> MGSSHHHHHHSSGLVPRGSHMQEQTAKEDVADSATSVGAIVSIEKAEKNFVITYASGKKAQISILNDHLFRYHLDPTGKFEEYPTPNDPKHVAKITAKTMADYGTQAFEQTNVTDSGNQFILENNGLKIIFEKESALMKVLDKKKNQVILEETAPLSFKNDKATQTLKQSSQENYFGGGTQNGRFTHKGTAIQIVNTNNWVDGGVASPNPFYWSTAGYGVVRNTWKPGNYDFGSHDPQTTTTTHEGTDFDAFYFFNDSSAGILKDYYELTGKPALMPEYGFYEAHLNAYNRDYWVKVAEGTAGAVKFEDGNFYKEYQPGDLGNLNGTLESLNGEKENYQFSARAVIDRYKKNDMPLGWFLPNDGYGAGYGQTDSLDGDVQNLKEFTDYAQANGVEVGLWTQSNLHPADPKNPKKGERDIAKEVSVAGVKALKTNVAWVGYGYSFGLNGVEDAANVFVKETDGAVRPM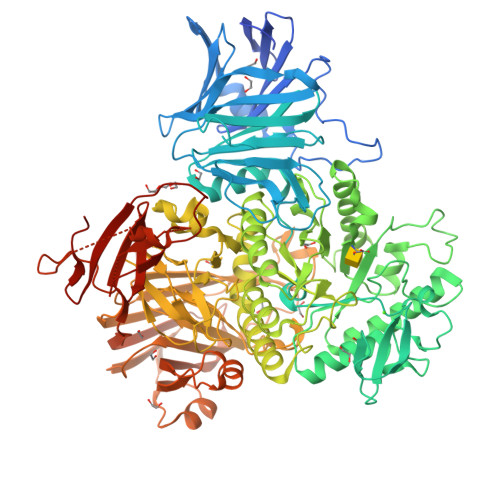IVSLDGWAGTQRHAGIWTGDQTGGQWEYIRFHIPTYIGTSLSGQPNVGSDMDGIFGGKNKEVNIRDFQWKTFTPVQLNMDGWGSNPKTPFAFDQEATDLNRAYLKLKSMMMPYNYSIAKESVDGLPMVRAMALEFPNEGTAYTKDSQYQYMWGPNLLVAPIYNGNQDEAGNSIRDGIYLPDEKQVWVDLFTGEKYQGGRVLNGVKTPLWKVPVFVKDGSIIPMTNPNNNPKEIQRDQRSFLIYPNGATSFNMYEDDGISTSYEAGQSATTKINSQGPKSNEKGDLTVTIEPTKGSYKDFVDERSTTLDLLASEAPESVTAMVGGTEVTLKQAANKEEFLAGTNLYYFDKEFQVNQYLSEASGEKLNQSALSVKLAKQSVTAKDVQITVKGFINKGTVDGGNTTVDDQLTIPANIAINEEKTTPSSLTLQWDQVTEATSYEVERDGTVFGNIQTNTATFDGFSFLSEHTFRVRAVGKNGVSEWSEPIKGKTQDDPYK ethyl 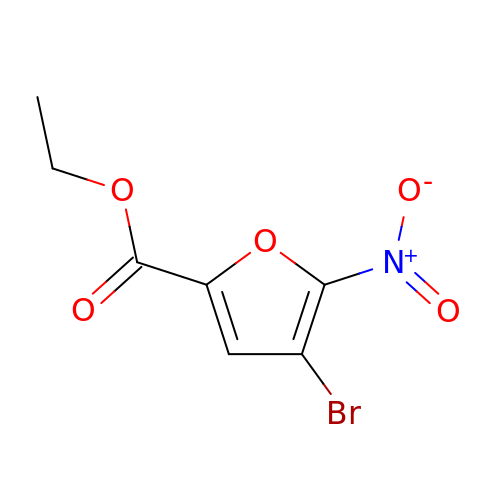4-bromanyl-5-nitro-furan-2-carboxylate | C7 H6 Br N O5 | ISDYKCYQNXYVMQ-UHFFFAOYSA-N>[2x]MSASLILDEYLKKT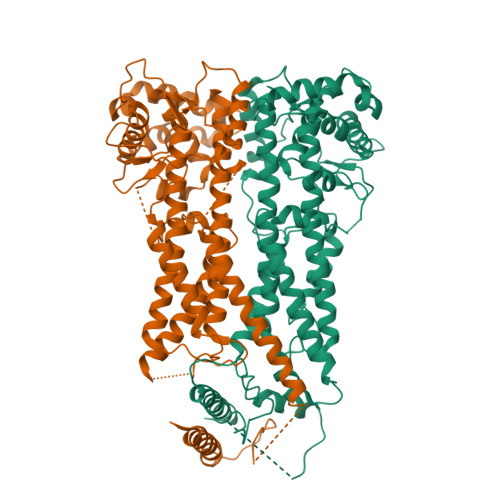ASAVLDVADSFEKIKGEIQSPEEAAALSVALYGAPPKPSASAVASIITGERTSLNDKYLSDNVLLKMSVARVGQENNRKRADQAADEIRTIMEDITGSLSGAYRQYSPLEEENKVHIGIMNNKTPSIVCGYYTMDTSISSEPLSLTDFQNPTVIANVTKRMESIFSKVDSARSTRFDAFVNGVANNMDIKSSIDWANMVENVIKLPDSTPNPCSVDTIVSRDASVVKTAVNDIYASVGKSYCRPATQLTFMSEIEKLRKAAVVCFEALMSDTRERAFVEFLFYVSFKEDASNTNSKLFVQNKLSSMSGNPRQPIKLVRRSAEETLFGLCFMFKVMPPEFMNCIFNFPTIPHSTQYHGLYGTCLTPLLRKYGSSFEKSWAHFEEILSERANAVKKFGVNDTRIDCLDAVANLTGPVYVLILDLVRTLSAQRSCSTKFLREIKENYLLWNRFVS The F-type ATP synthase (F1Fo-ATP synthase) is responsible for generating most of the cellular adenosine triphosphate (ATP) from adenosine diphosphate (ADP) and inorganic phosphate through rotary catalysis. In eukaryotes, ATP synthases are found in the inner mitochondrial membrane. The type III ATP synthase was detected in ciliates where it induces tubulation of the cristae membranes. In this study, we present the cryo-EM structures of the type III ATP synthase dimer and tetramer with associated lipids from the model organism Tetrahymena thermophila in complex with the natural inhibitor IF1.

Using masked refinements, the resolution of different regions reached 2.5–3.1 Å, allowing de novo modelling.

>MLLVKAVKVLVMGGCMLPIAFGALGTGVLFAGFNVALSRNPEETESLFNNTLMGFALIETFIFMSIGLGFFVLFAA[10x];> MFTRFVTQPTLLTQTQRALFSALTKKQKMEVTLRTPYKEYLANFDGFSRITAKTNEASLVIQNKTPASLYVLPPGPLKIRFTSEVKNVSGDFLHTGGWVIVHADNTCEINVMDLFDRKEVRADQFEKGNIQDLDTLAGKYAAKSRKSTVRLFTKATTQ;> MCIEFAFKKAGIPIVRNFLHSTEGVIYGLPQRVQRNLAINYTVKQYKEGKAVSAKTIKTLQEAFPSKGDTK;> MFGLASKGFINTSLVMVPQMNFGANLKQLKIRMKAIGSIKKITKAMKMVAASKMKAETSRLENGRNFAVGSVQKMLENESYVQKKKSTTAPKSTLLVPITSDKGLCGSVNSSIVREVKRLALNNRSAFGLLPVGEKGSSGLSRPFPDLLKSSIVNIQNVNFPTAAAIAHQVSTQGAGYDQVTLIYNHFKNAISYVVKHQELLPRAQFLNLFKYVTRHEAVEPELEYSKNYFFELYMASSVYNALLNSSASEQASRMNAMENASKNAGEILSKLTLDYNKARQAKITMELIEIISGASIV>PAVLELEGKKWRVENQENVSNLVIEDTELKQVAYIYKCVNTTLQIKGKINSITVDNCKKLGLVFDDVVGIVEIINSKDVKVQVMGK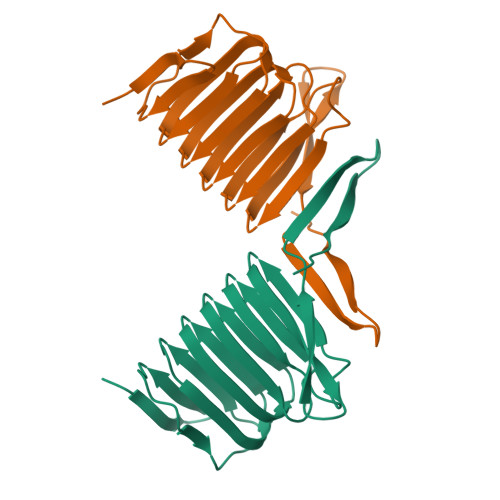VPTISINKTDGCHAYLSKNSLDCEIVSAKSSEMNVLIPTEGGDFNEFPVPEQFKTLWNGQKLVTTVTEIAG[4x]>[2x]MQTEHVILLNAQGVPTGTLEKYAAHTADTRLHLAFSSWLFNAKGQLLVTRRALSKKAWPGVWTNSVCGHPQLGESNEDAVIRRCRYELGVEITPPESIYPDFRYRATDPSG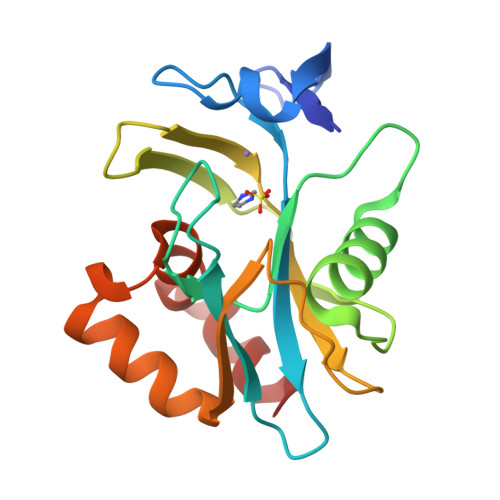IVENEVCPVFAARTTSALQINDDEVMDYQWCDLADVLHGIDATPWAFSPWMVMQATNREARKRLSAFTQLKL> HGSPVDICTAKPRDIPMNPMCIYRSPEKKATEDEGSEQKIPEATNRRVWELSKANSRFATTFYQHLADSKNDNDNIFLSPLSISTAFAMTKLGACNDTLQQLMEVFKFDTISEKTSDQIHFFFAKLNCRLYRKANKASKLVSANRLFGDKSLTFNETYQDISELVYGAKLQPLDFKENAEQSRAAINKWVSNKTEGRITDVIPSEAINELTVLVLVNTIYFKGLWKSKFSPENTRKELFYKADGESCSASMMYQEGKFRYRRVAEGTQVLELPFKGDDITMVLILPKPEKSLAKVEKELTPEVLQEWLDELEEMMLCVHMPRFRIEDGFSLKEQLQDMGLVDLFSPEKSKLPGIVAEGRDDLYVSDAFHKAFLEVNEEGSEAAASTAVVIAGRSLNPNRVCFKANRPFLVFIREVPLNTIIFMGRVANPCVK;> HGSPVDICTAKPRDIPMNPMCIYRSPEKKATEDEGSEQKIPEATNRRVWELSKANSRFATTFYQHLADSKNDNDNIFLSPLSISTAFAMTKLGACNDTLQQLMEVFKFDTISEKTSDQIHFFFAKLNCRLYRKANKSSKLVSA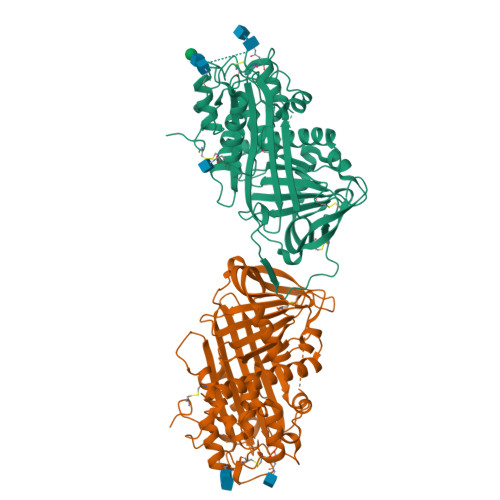NRLFGDKSLTFNETYQDISELVYGAKLQPLDFKENAEQSRAAINKWVSNKTEGRITDVIPSEAINELTVLVLVNTIYFKGLWKSKFSPENTRKELFYKADGESCSASMMYQEGKFRYRRVAEGTQVLELPFKGDDITMVLILPKPEKSLAKVEKELTPEVLQEWLDELEEMMLVVHMPRFRIEDGFSLKEQLQDMGLVDLFSPEKSKLPGIVAEGRDDLYVSDAFHKAFLEVNEEGSEAAASTAVVIAGRSLNPNRVTFKANRPFLVFIREVPLNTIIFMGRVANPCVK> E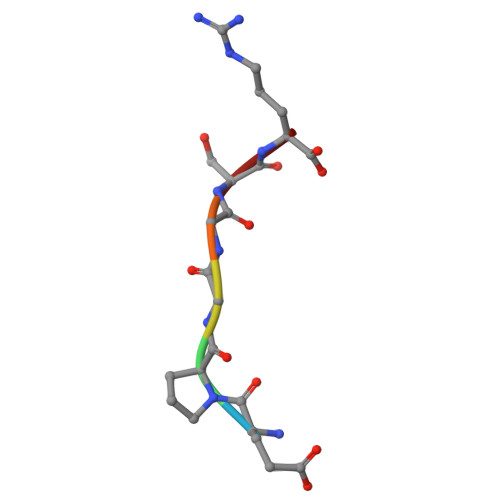PGGSR>XGEIAQALKEIAKALKEIAYALKEIAQALKGX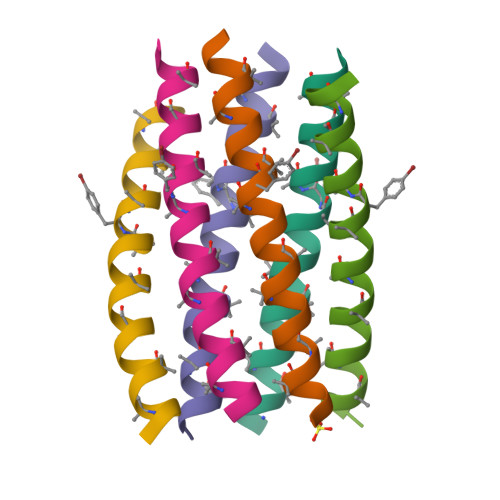[6x]>[2x]MDLTVEPNLHSLITSTTHKWIFVGGKGGVGKTTSSCSIAIQMALSQPNKQFLLISTDPAHNLSDAFGEKFGKDARKVTGMNNLSCMEIDPSAALKDMNDMAVSRANNNGSDGQGDDLGSLLQGGALADLTGSIPGIDEALSFMEVMKHIKRQEQDEGETFDTVIFDTAPTGHTLRFLQLPNTLSKLLEKFGEITNKLGPMLNSFMGAGNVDISGKLNELKANVETIRQQF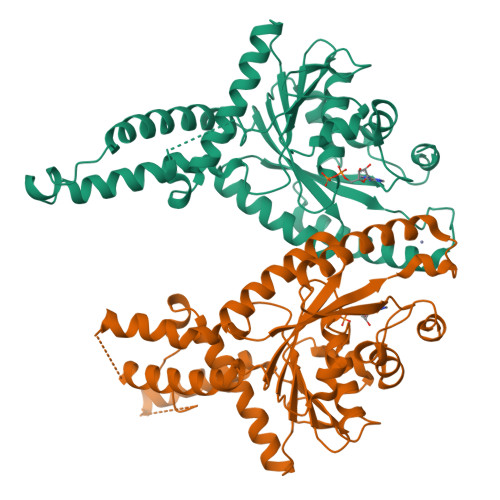TDPDLTTFVCVCISEFLSLYETERLIQELISYDMDVNSIIVNQLLFAENDQEHNCKRCQARWKMQKKYLDQIDELYEDFHVVKMPLCAGEIRGLNNLTKFSQFLNKEYNPITDGKVIYELEDKELEHHHHHH> MYVYKRDGRKEPVQFDKITARISRLCYGLDPKHIDAVKVTQRIISGVYEGVTTIELDNLAAETCAYMTTVHPDYATLAARIAISNLHKQTTKQFSKVVEDLYRYVNAATGKPAPMISDDVYNIVMENKDKLNSAIVYDRDFQYSYFGFKTLERSYLLRINGQVAERPQHLIMRVALGIHGRDIEAALETYNLMSLKYFTHASPTLFNAGTPKPQMSSCFLVAMKEDSIEGIYDTLKECALISKTAGGIGLHIHNIRSTGSYIAGTNGTSNGLIPMIRVFNNTARYVDQGGNKAPGAFALYLEPWHADIFDFIDIRKNHGKEEIRARDLFPALWIPDLFMKRVEENGTWTLFSPTSAPGLSDCYGDEFEALYTRYEKEGRGKTIKAQKLWYSILEAQTETGTPFVVYKDACNRKSNQKNLGVIKSSNLCCEIVEYSAPDETAVCNLASVALPAFIETSEDGKTSTYNFKKLHEIAKVVTRNLNRVIDRNYYPVEEA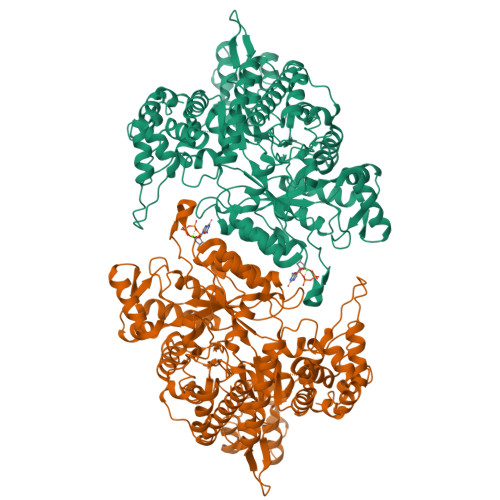RKSNMRHRPIALGVQGLADTFMLLRLPFDSEEARLLNIQIFETIYHASMEASCELAQKDGPYETFQGSPASQGILQFDMWDQKPYGMWDWDTLRKDIMKHGVRNSLTMAPMPTASTSQILGYNECFEPVTSNMYSRRVLSGEFQVVNPYLLRDLVDLGIWDEGMKQYLITQNGSIQGLPNVPQELKDLYKTVWEISQKTIINMAADRSVYIDQSHSLNLFLRAPTMGKLTSMHFYGWKKGLKTGMYYLRTQAASAAIQFTIDQKIADQATENVADISNLKRPSYMPSSASYAASDFVPAAVTANATIPSLDSSSEASREASPAPTGSHSLTKGMAELNVQESKVEVPEVPAPTKNEEKAAPIVDDEETEFDIYNSKVIACAIDNPEACEMCSG>AYAQWVIIIIHNVGSKDVKIKNLKPSWGKLHADGDKDTEVSASKYEGTVIKPDEKLQINACGRSDAAEGTTGTFDLVDPADGDKQVRHFYWDCPWGSKTNTWTVSGSNTKWMIEYSGQNLDSGALGTITVDTLKK[26x];>QAGDTLNDVIQDPTRRNKLINDNNLLKGIIMGRDGPVPSSRELIVRPDTLRAIINNRATIETTTMEAEFTETLMESNYNSASVKVSAPFITANSEYSESSSFKNTETEKSMYTSSRYLFPQGRIDFTTPDSGFDDVIKLSPQFTSGVQAALAKATGTEKREALQNLFQEYGHVFRTKVHIGGVLSAHTMETFSRSENETEVKQDVKAGLEGAVKGWGGGATAGHGNTQGTITTSQNRKLNVKYIVNGGDYTKIQNTEEWVASTNQSEHWRVIEVTEVTAVADLLPQPIRGQVKDLLKPLLGKWVDVEKVPGLESLPVSVYRPKGAIPAGWFWLGDTADASKALLVKPTLPARSGRNPALTSLHQGSGMTEQPFVDLPQYQYLSTYFGSFAHDTPPGSTLRGLRPDHVLPGRYEMHGDTISTAVYVTRPVDVPFPEDECFDLKSLVRVKLPGSGNPPKPRSALKKSMVLFDSGEK[12x];> SQAGDTLNDVIQDPTRRNKLINDNNLLKGIIMGRDGPVPSSRELIVRPDTLRAIINNRATIETTTMEAEFTETLMESNYNSASVKVSAPFITANSEYSESSSFKNTETEKSMYTSSRYLFPQGRIDFTTPDSGFDDVIKLSPQFTSGVQAALAKATGTEKREALQNLFQEYGHVFRTKVHIGGVLSAHTMETFSRSENETEVKQDVKAGLEGAVKGWGGGATAGHGNTQGTITTSQNRKLNVKYIVNGGDYTKIQNTEEWVASTNQSEHWRVIEVTEVTAVADLLPQPIRGQVKDLLKPLLGKWVDVEKVPGLESLPVSVYRPKGAIPAGWFWLGDTADASKALLVKPTLPARSGRNPALTSLHQGSGMTEQPFVDLPQYQYLSTYFGSFAHDTPPGSTLRGLRPDHVLPGRYEMHGDTISTAVYVTRPVDVPFPEDECFDLKSLVRVKLPGSGNPPKPRSALKKSMVLFDSGEK

To gain further insight into the structural conversions in pore formation, we chose pleurotolysin (Ply), a MACPF protein consisting of two components, PlyA and PlyB, from Pleurotus ostreatus. Previous studies have shown that PlyA binds membranes and is required to recruit the pore-forming MACPF protein PlyB to the membrane surface. PlyA and PlyB together form relatively small and regular pores in liposomes. The membrane attack complex/perforin-like family (MACPF) proteins form the largest superfamily of pore-forming proteins identified to date.

The images were analysed by the single particle approach, following the method developed for the CDC pneumolysin. This allowed us to sort the pore views by symmetry, enabling determination of an 11 Å resolution cryo-EM map of a liposome-embedded 13-fold pleurotolysin pore from 8,770 views. In the pore map, the position of PlyB is clearly recognizable in the upper part of each subunit, while the V-shaped density at the base of each asymmetric unit accommodates two PlyA molecules. The core of the MACPF domain undergoes a massive opening but does not collapse as in CDCs. In this pore, the central β-sheet has straightened and opened by ∼70°, as measured from the fitting, and TMH1 and TMH2 are fully unwound into β-hairpins to form a β-barrel spanning the membrane bilayer. The pore channel is thus formed by a 52-stranded β-barrel that is 80 Å in inner diameter and over 100 Å in height. The PlyB C-terminal trefoil sits in the cavity formed by a V-shaped wedge of density contacting the membrane. This density can be accounted for by two PlyA molecules, revealing a tridecameric PlyB/2xPlyA pore assembly. The resulting fit of 26 PlyA and 13 PlyB subunits had a cross-correlation coefficient of 0.8 with the map which includes part of the membrane as measured in Chimera.TRAP has proved a useful building block for construction of artificial nanostructures. The wild‐type protein forms a ring‐shaped assembly comprising 11 identical monomers. We have shown that cysteine‐modified variants of the trp RNA binding attenuation protein, assemble into cage‐like structures with Au(I) or Hg(II), called TRAP‐cage, disassembly of which can be induced by thiol‐ or phosphine‐containing compounds. Here, we report variants of TRAP which can assemble into TRAP‐cages mediated by Co(II) or Zn(II).

Based on the crystal structure of wild‐type TRAP, a histidine residue was introduced at position 33 of the TRAPK35C variant, yielding TRAPS33H/K35C, where the histidine and cysteine residues are located at i and i+2 positions of the β‐sheet motif around the rim of the ring‐shaped structure. The cysteine residue at position 35 of TRAPS33H/K35C was further changed to histidine, resulting in another variant, TRAPS33H/K35H, possessing a pair of imidazole ligands. When the TRAPS33H/K35H protein was mixed with Co(II) or Zn(II), it showed the formation of pseudospherical cages with a diameter of ≈22 nm, similar to TRAP Au(I) 24‐cage. We constructured a number of cages named as follows: Cages made with Zn(II) (TRAPK35C‐Zn(II)‐cages); TRAPS33H/K35H with either Co(II) or Zn(II) (TRAPS33H/K35H‐Co(II) or ‐Zn(II)‐cages); TRAPS33H/K35C with Zn(II) (TRAPS33H/K35C‐Zn(II)‐cages). To verify our designs, we solved the structures of TRAPS33H/K35H‐Zn(II)‐cage, TRAPS33H/K35H‐Co(II)‐cage, and TRAPK35C‐Zn(II)‐cages using cryoEM single particle reconstruction (see Methods for sample preparation and Figures S2–S4 for analysis pipelines). The resulting structures showed that these cages are mainly composed of 24 TRAP rings, and the overall shape and bonding network between adjacent rings is retained when compared to the TRAPAu(I) 24‐cage. They form two chiral cages, and each ring forms two metal‐mediated bridges with each neighbor. In the structure of TRAPS33H/K35H‐Co(II)‐cage, every bridge has in its center one ion in close proximity to the histidine residues introduced in positions 33 and 35 as expected. However, a closer analysis revealed that the coordination geometry is unlikely to be a perfect tetrahedron but rather a distorted one or an octahedron formed by 4 histidine ligands from the protein and 2 bonds with other ligands such as water molecules (which are not visible due to limited resolution). TRAP‐cages that possess only histidine ligands, TRAPS33H/K35H‐Co(II) cages, and TRAPS33H/K35H‐Zn(II) cages, almost completely disassembled in the presence of 35 µM EDTA (1 equivalent to TRAP monomer). TRAPS33H/K35H‐Co(II) and Zn(II)‐cages were more sensitive to pH, disassembling completely at pHs below 4–6 and above 8–10.

>[264x]MYTNSDFVVIKALEDGVNVIGLTRGADTRFHHHEHLDKGEVLIAQFTEHTSAIKVRGKAYIQTRHGVIESEGKK>SVDHGFLVTRHSQTIDDPQCPSGTKILYHGYSLLYVQGNERAHGQDLGTAGSCLRKFSTMPFLFCNINNVCNFASRNDYSYWLSTPEPMPMSMAPITGENIRPFISRCAVCEAPAMVMAVHSQTIQIPPCPSGWSSLWIGYSFVMHTSAGAEGSGQALASPGSCLEEFRSAPFIECHGRGTCNYYANAYSFWLATIERSEMFKKPTPSTLKAGELRTHVSRC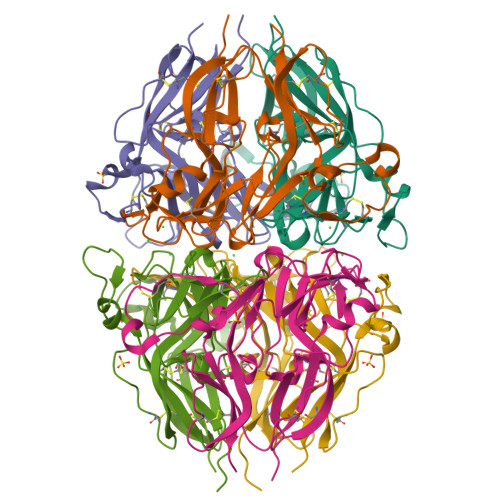QVCMRRT[6x]>GRKKIQISRILDQRNRQVTFTKRKFGLMKKAYELSVLCDCEIALIIFNSANRLFQYASTDMDRVLLKYTEYSEPHESRTNTDILETLKRRGIG[2x];> TLLSPKGSISEETKQ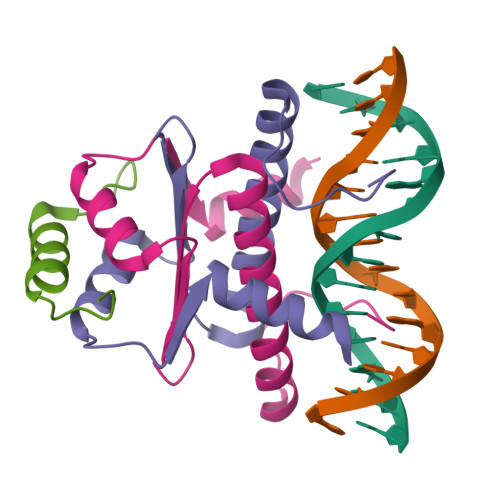KLKSAILSAQSAANVRKESL> FSGSEATAAILSRAPWSLQSVNPGLKTNSSKEPKFTKCRSPERETFSCHWTDEVHHGTKNLGPIQLFYTRRNTQEWTQEWKECPDYVSAGENSCYFNSSFTSIWIPYCIKLTSNGGTVDEKC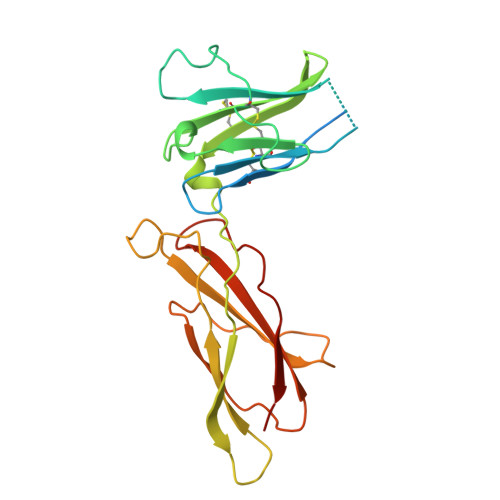FSVDEIVQPDPPIALNWTLLNVSLTGIHADIQVRWEAPRNADIQKGWMVLEYELQYKEVNETKWKMMDPILTTSVPVYSLKVDKEYEVRVRSKQRNSGNYGEFSEVLYVTLPQMS Alanine racemase (Alr, EC 5.1.1.1) is a fold-type III pyridoxal 5’-phosphate (PLP)-dependent enzyme that catalyzes the reversible racemization of L-Ala and D-Ala. D-Ala is one of the key building blocks of peptidoglycan network, an elastic polymer layer consisting of sugars and amino acids that forms the bacteria cell wall, protecting cell against osmotic pressure and attack from L-amino acids targeted peptidases. However, the alr gene encodes an anabolic alanine racemase Alr, it is expressed constitutively at low level and essential for providing abundant D-Ala for peptidoglycan biosynthesis. T. tengcongensis MB4 contains two annotated alanine racemase genes MBalr1 (AAM24437.1) and MBalr2 (AAM25327.1).

In order to understand the biochemical properties of AlrTt, especially the role of the non-conserved residue Gln360 in alanine racemization, we determined the crystal structure of AlrTt in complex with L-Ala at 2.7 Å resolution, and investigated its racemase activity by saturation mutagenesis of Gln360. Like typical alanine reacemase, a homo-dimer of AlrTt was found in one asymmetric unit. Each monomer covers full-length AlrTt (Val1-Lys383), it contains an N-terminal eight-stranded α/β barrel domain (residues 1–244) and a C-terminal extended β-strand domain (residues 245–383). Although we co-crystallized AlrTt with PLP and L-Ala, only L-Ala and the phosphate group of PLP were observed in the active site of AlrTt, the pyridine ring is not interpreted due to lack of clear electron density. First, side chain of the key catalytic base Lys40 forms a hydrogen bond with carboxyl group of Asp317’ (2.6 Å), disrupted the covalent bond with pyridine ring that is necessary for forming the internal aldimine. However, these interactions are disrupted or much weaker in AlrTt: His205-Arg224 (4.5Å), Arg224-His168 (3.5Å), His168-Tyr268’ (3.0 Å). Thus, side chain of Arg224 is not properly coordinated by His205 and His168 to adopt an optimal orientation for stabilizing the N1 atom of the pyridine ring. The short side chain of Gln360 disrupted the hydrogen bond with OP2 (4.0 Å), which is highly conserved in other bacterial alanine racemase. One L-Ala molecule is positioned in the active site pocket by hydrogen bonds with main chain nitrogen of Met316’ (2.6 Å), OH of inner layer residue Tyr287’ (2.8 Å) and Tyr268’ (2.7 Å). Presence of Gln360 and conformational changes of Lys40, Arg224 and Tyr44 destroy the hydrogen bonding interactions necessary for stabilizing the pyridine ring and phosphate group, result in weaker PLP binding and low racemase activity of AlrTt.

>VKFDGVRPTRVEVYLDAITHNFREIKKIVGKNVKIMAVIKGDAYGHGASYVAKFLEKEGVDYFGVATTEEALELREKGIKTPILIFGYTPPTQLRQIVKHDLTQTVYDIKYAKELEKESLKQNKRAKVHIKIDTGLGRIGYIDFDLAQKEILEMANMRGLILEGIYSHFAAASEDDRDYCKEQFDKFMNLISSLEKKRLKIPLKHIANAAAILNLNYSHLDMVRPGIILFGAYPSKRVERKVELRETLRFTTRVVHLKDVPAGFFIGYGKSFVTKRKSVIATIPVGYADGLDRRLSNNYKLLLKGKYVPIVGRVCMDQCMIDVTDVEGVEIGDEVVIIGTQNNETVSVESMADKIETIPQEVFSRISRRVPRVYFYDGIKIGEVNYLK[2x]>[2x]MNKLAVLYAEHIATLQKRTREIIERENLDGVVFHSGQAKRQFLDDMYYPFKVNPQFKAWLPVIDNPHCWIVANGTDKPKLIFYRPVDFWHKVPDEPNEYWADYFDIELLVKPDQVEKLLPYDKARFAYIGEYLEVAQALGFELMNPEPVMNFYHYHRAYKTQYELACMREANKIAVQGHKAARDAFFQGKSEFEIQQAYLLATQHSENDTPFGNIVALNENCAILHYTHFDRVAPATHRSFL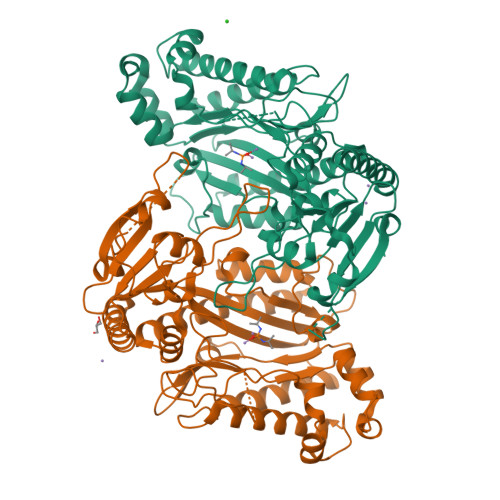IDAGANFNGYAADITRTYDFTGEGEFAELVATMKQHQIALCNQLAPGKLYGELHLDCHQRVAQTLSDFNIVNLSADEIVAKGITSTFFPHGLGHHIGLQVHDVGGFMADEQGAHQEPPEGHPFLRCTRKIEANQVFTIEPGLYFIDSLLGDLAATDNNQHINWDKVAELKPFGGIRIEDNIIVHEDSLENMTRELELD>[2x]SNAMQRRLERFDAKLVQSGLDALLVTGQNNIYYLTDFWGTNATVFITKNRRLFLTDSRYTLIAKQSVHGFDIIESKDPLKDIVKFVEVDKLETIGFDNQVSFAY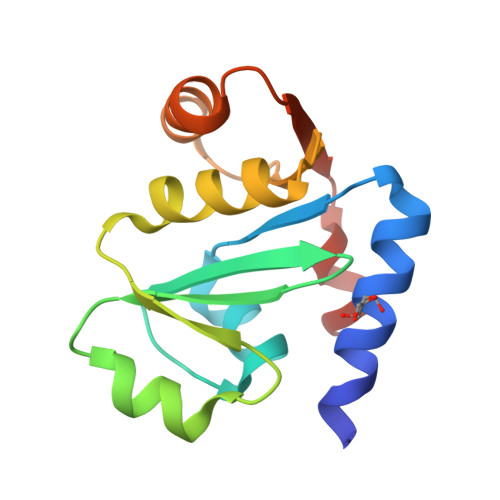YQALQAIFEGYTLSPQTNFMEELRMIK> MGPLWLDVAGYELSAEDRAILAHPTVGGVILFGRNYHDNQQLLALNKAIRQAAARPILIGVDQEGGRVQRFREGFSRIPPAQYYARAENGVELAEQGGWLMAAELIAHDVDLSFAPVLDMGFACKAIGNRAFGEDVQTVLKHSSAFLRGMKAVGMATTGKHFPGHGAVIADSHLETPYDERETIAQDMAIFRAQIEAGVLDAMMPAHVVYPHYDAQPASGSSYWLKQVLREELGFKGIVFSDDLSMEGAAVMGGPVERSHQALVAGCD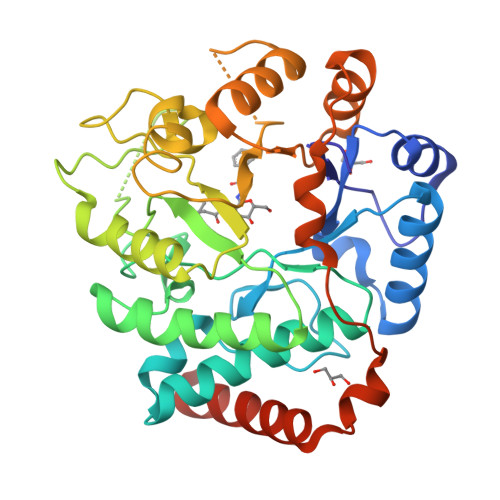MILICNKREAAVEVLDNLPIMEVPQAEALLKKQQFSYSELKRLERWQQASANMQRLIEQFSEHHHHHHHHHH(3S,4S)-4-({[4-methoxy-3-(3-methoxypropoxy)benzoyl](propan-2-yl)amino}methyl)pyrrolidin-3-yl 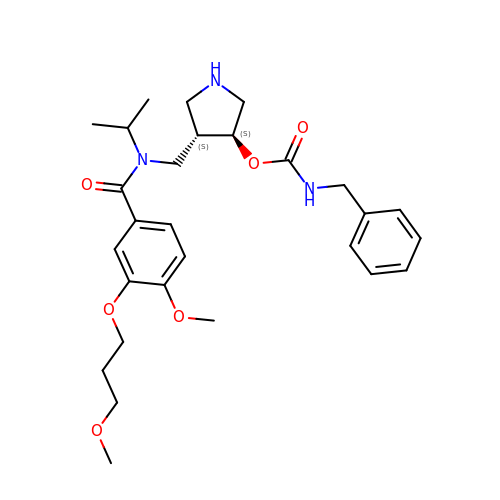benzylcarbamate | C28 H39 N3 O6 | WGHJKYWWSVIRLL-JYFHCDHNSA-N N-{[(3S,4S)-4-benzylpyrrolidin-3-yl]methyl}-4-methoxy-3-(3-methoxypropoxy)-N-(propan-2-yl)benzamide | C27 H38 N2 O4 | 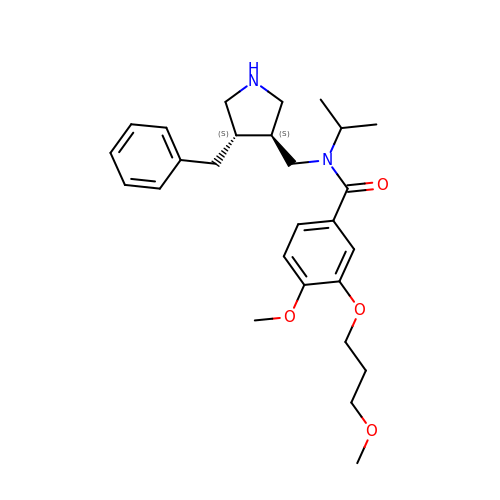PHCCFIGNVNPMML-RPWUZVMVSA-N>KKRVFTFGKGRSEGNRDMKSLLGGKGANLAEMSSIGLSVPPGLTISTEACEEYQQNGKSLPPGLWDEISEGLDYVQKEMSASLGDPSKPLLLSVRSGAAISMPGMMDTVLNLGLNDEVVAGLAGKSGARFAYDSYRRFLDMFGNVVMGIPHSLFDEKLEQMKAEKGIHLDTDLTAADLKDLVEKYKNVYVEAKGEKFPTDPKKQLELAVNAVFDSWDSPRANKYRSINQITGLKGTAVNIQSMVFGNMGNTSGTGVLFTRNPSTGEKKLYGEFLINAQGEDVVAGIRTPEDLGTMETCMPEAYKELVENCEILERHYKDMMDIEFTVQENRLWMLQCRTGKRTGKGAVRIAVDMVNEGLIDTRTAIKRVETQHLDQLLHPQFEDPSAYKSHVVATGLPASPGAAVGQVCFSAEDAETWHAQGKSAILVRTETSPEDVGGMHAAAGILTARGGMTSHAAVVARGWGKCCVSGCADIRVNDDMKIFTIGDRVIKEGDWLSLNGTTGEVILGKQLLAPPAMSNDLEIFMSWADQARRLKVMANADTPNDALTARNNGAQGIGLCRTEHMFFASDERIKAVRKMIMAVTPEQRKVALDLLLPYQRSDFEGIFRAMDGLPVTIRLLDPPLHEFLPEGDLEHIVNELAVDTGMSADEIYSKIENLSEVNPMLGFRGCRLGISYPELTEMQVRAIFQAAVSMTNQGVTVIPEIMVPLVGTPQELRHQISVIRGVAANVFAEMGVTLEYKVGTMIEIPRAALIAEEIGKEADFFSFGTNDLTQMTFGYSRDDVGKFLQIYLAQGILQHDPFEVIDQKGVGQLIKMATEKGRAANPSLKVGICGEHGGEPSSVAFFDGVGLDYVSCSPFRVPIARLAAAQVIV[2x]

Here, the rate limiting regeneration of the primary CO2 acceptor phosphoenolpyruvate (PEP) is catalyzed by the multi-domain protein pyruvate phosphate dikinase (PPDK). Previous studies emphasize that PPDK has a modular structure consisting of distinct substrate binding domains for PEP/pyruvate at the C-terminus (PBD) and for nucleotides ATP/AMP at the N-terminus (NBD, aa 1–340). A central domain (CD, aa 380–515) catalyzing the phosphoryl group transfer from ATP to pyruvate–or from PEP to AMP–via a phospho-histidine intermediate mediates a catalytic cross-talk between the distant substrate binding domains. Distinct conformational states resolved in crystal structures from maize and the non-plant organisms Clostridium symbiosum and Trypanosoma brucei suggest that the phosphoryl group transfer in the catalytic cycle is accompanied by a large swiveling motion of the CD from a position next to the NBD to a position facing the PBD (~110° and 45 Å).

The main difference is found in the NBD of both monomers with the A monomer reflecting an open conformation and the B monomer reflecting a closed conformation of this domain. Superimposition of the NBD subdomains highlights that NBD1 is reoriented by a large motion of about 40° around a hinge region consisting of two short peptide linkers formed by residues 112–115 and 195–200 towards NBD3. At the same time, NBD2 is displaced by about 40° to accommodate for the new position of NBD1. The hinge motion of NBD1 and NBD2 results in the closing of the large cleft formed in the open configuration of the PPDK monomer. This cleft is no longer accessible in the closed form of the PPDK monomer. Yet, both monomers show electron density in the PBD for the co-crystallized substrate PEP. Besides, the NBD of monomer B exhibits additional density in both the mFo − DFc difference map and the feature enhanced maps (FEM, see methods section) probably reflecting a bound adenine nucleotide. The overall shape of this additional density is consistent with structural requirements and binding mode of adenine nucleotides in other nucleotide-binding proteins with the ATP-grasp fold1617. However, since the molecular identity of the bound compound was not fully resolved at the present resolution, no compound was placed in this density in the deposited structure. The presence of two structurally distinct conformations of the PPDK monomer (NBD open versus closed) within a single crystal structure may suggest that these structural asymmetries reflect functional asymmetries in substrate binding and/or catalytic turnover in the individual subunits of the PPDK dimer.>RGSHMEKLAKNKVISIDAGRKYFTLNQLKRIVDKASELGYSDVHLLLGNDGLRFLLDDMTITANGKTYASDDVKKAIIEGTKAYYDDPNGTALTQAEVTELIEYAKSKDIGLIPAINSPGHMDAMLVAMEKLGIKNPQAHFDKVSKTTMDLKNEEAMNFVKALIGKYMDFFAGKTKIFNFGTDEYANDATSAQGWYYLKWYQLYGKFAEYANTLAAMAKERGLQPMAFNDGFYYEDKDDVQFDKDVLISYWSKGWWGYNLASPQYLASKGYKFLNTNGDWYYILGQKPEDGGGFLKKAIENTGKTPFNQLASTKYPEVDLPTVGSMLSIWADRPSAEYKEEEIFELMTAFADHNKDYFRANYNALREELAKIPTNLEGYSKESLEALDAAKTALNYNLNRNKQAEL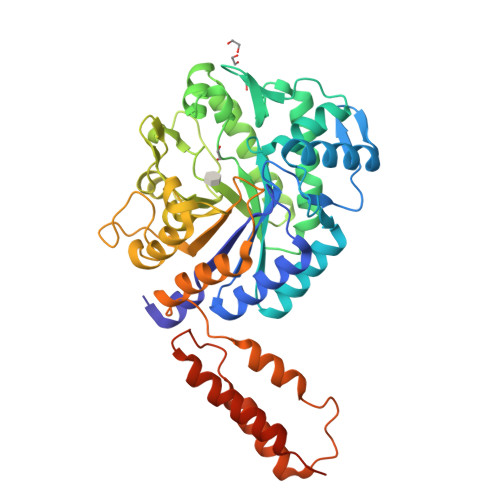DTLVANLKAALQGLKPAVTHSGSLDENEVAANVETRP[4x]> MKTEWPELVGKSV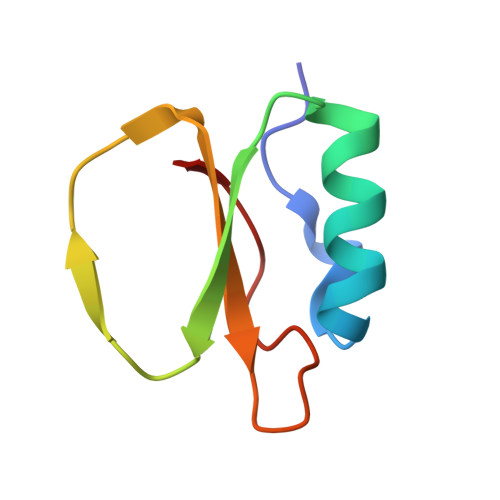EEAKKVILQDKPAAQIIVLPVGTIVTYEYRIDRVRLFVDRLDNIAQVPRVG>[2x]MEEPEEPADSGQSL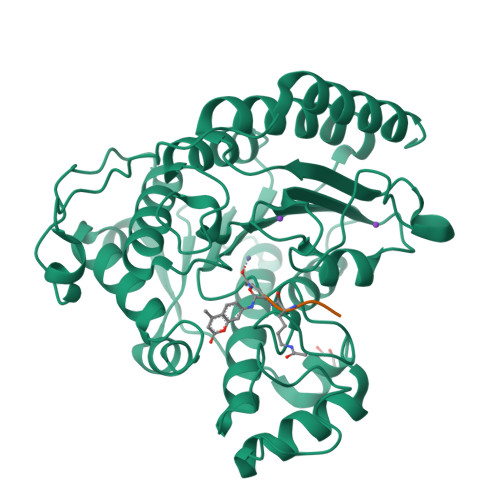VPVYIYSPEYVSMCDSLAKIPKRASMVHSLIEAYALHKQMRIVKPKVASMEEMATFHTDAYLQHLQKVSQEGDDDHPDSIEYGLGYDCPATEGIFDYAAAIGGATITAAQCLIDGMCKVAINWSGGWHHAKKDEASGFCYLNDAVLGILRLRRKFERILYVDLDLHHGDGVEDAFSFTSKVMTVSLHKFSPGFFPGTGDVSDVGLGKGRYYSVNVPIQDGIQDEKYYQNCESVLKEVYQAFNPKAVVLQLGADTIAGDPMCSFNMTPVGIGKCLKYILQWQLATLILGGGGFNLANTARCWTYLTGVILGKTLSSEIPDHEFFTAYGPDYVLEITPSCRPDRNEPHRIQQILNYIKGNLKHVVIEGRGSHHHHHH;>[2x]XRHKK>[4x]MDLKGGESMVDWKLMQEIIEAPGVSGYEHLGIRDIVVDVLKEVADEVKVDKLGNVIAHFKGSSPRIMVAAHMDKIGVMVNHIDKDGYLHIVPIGGVLPETLVAQRIRFFTEKGERYGVVGVLPPHLRRGQED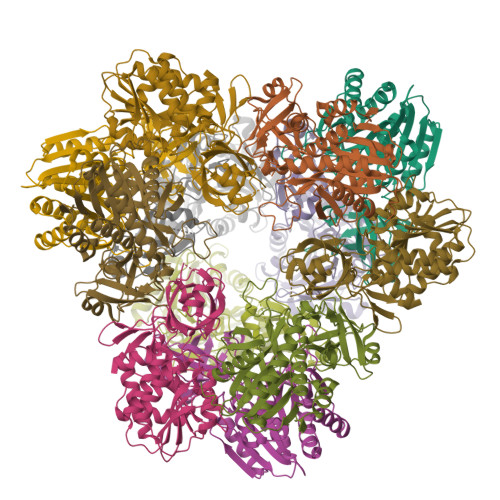KGSKIDWDQIVVDVGASSKEEAEEMGFRVGTVGEFAPNFTRLNEHRFATPYLDDRICLYAMIEAARQLGDHEADIYIVGSVQEEVGLRGARVASYAINPEVGIAMDVTFAKQPHDKGKIVPELGKGPVMDVGPNINPKLRAFADEVAKKYEIPLQVEPSPRPTGTDANVMQINREGVATAVLSIPIRYMHSQVELADARDVDNTIKLAKALLEELKPMDFTP>MSETFTKGMARNIYFGGSVFFILLFLALTYHTEKTLPERTNEAAMSAAVVRGKLVWEQNNCVGCHTLLGEGAYFAPELGNVVGRRGGEEGFNTFLQAWMKIQPLNVPGRRAMPQFHLSEGQVDDLAEFLKWSSKIDTNQWPPNKEG[2x];>MMSPNGSLKFASQAVAKPYFVFALILFVGQILFGLIMGLQYVVGDFLFPAIPFNVARMVHTNLLIVWLLFGFMGAAYYLVPEESDCELYSPKLAWILFWVFAAAGVLTILGYLLVPYAGLARLTGNELWPTMGREFLEQPTISKAGIVIVALGFLFNVGMTVLRGRKTAISMVLMTGLIGLALLFLFSFYNPENLTRDKFYWWWVVHLWVEGVWELIMGAILAFVLVKITGVDREVIEKWLYVIIAMALISGIIGTGHHYFWIGVPGYWLWLGSVFSALEPLPFFAMVLFAFNTINRRRRDYPNRAVALWAMGTTVMAFLGAGVWGFMHTLAPVNYYTHGTQLTAAHGHMAFYGAYAMIVMTIISYAMPRLRGIGEAMDNRSQVLEMWGFWLMTVAMVFITLFLSAAGVLQVWLQRMPADGAAMTFMATQDQLAIFYWLREGAGVVFLIGLVAYLLSFRRGKAAA[2x];>MPFGKPLVGTLLASLTLLGLATAHAKDDMKAAEQYQGAASAVDPAHVVRTNGAPDMSESEFNEAKQIYFQRCAGCHGVLRKGATGKPLTPDITQQRGQQYLEALITYGTPLGMPNWGSSGELSKEQITLMAKYIQHTPPQPPEWGMPEMRESWKVLVKPEDRPKKQLNDLDLPNLFSVTLRDAGQIALVDGDSKKIVKVIDTGYAVHISRMSASGRYLLVIGRDARIDMIDLWAKEPTKVAEIKIGIEARSVESSKFKGYEDRYTIAGAYWPPQFAIMDGETLEPKQIVSTRGMTVDTQTYHPEPRVAAIIASHEHPEFIVNVKETGKVLLVNYKDIDNLTVTSIGAAPFLHDGGWDSSHRYFMTAANNSNKVAVIDSKDRRLSALVDVGKTPHPGRGANFVHPKYGPVWSTSHLGDGSISLIGTDPKNHPQYAWKKVAELQGQ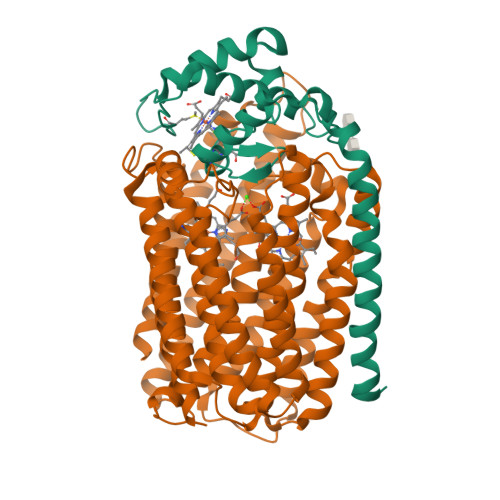GGGSLFIKTHPKSSHLYVDTTFNPDARISQSVAVFDLKNLDAKYQVLPIAEWADLGEGAKRVVQPEYNKRGDEVWFSVWNGKNDSSALVVVDDKTLKLKAVVKDPRLITPTGKFNVYNTQHDVY[2x]> HHHHHHMAQDRKKVLVLGAGYAGLQTVTKLQKAISTEEAEITLINKNEYHYEATWLHEASAGTLNYEDVLYPVESVLKKDKVNFVQAEVTKIDRDAKKVETNQGIYDFDILVVALGFVSETFGIEGMKDHAFQIENVITARELSRHIEDKFANYAASKEKDDNDLSILVGGAGFTGVSFLGELTDRIPELCSKYGVDQ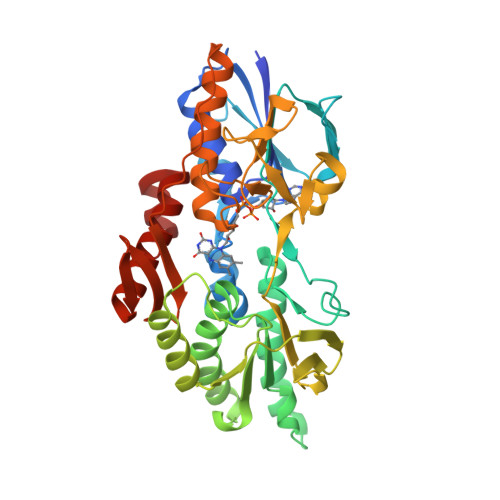NKVKITCVEAAPKMLPMFSEELVNHAVSYLEDRGVEFKIATPIVACNEKGFVVEVDGEKQQLNAGTSVWAAGVRGSKLMEESFEGVKRGRIVTKQDLTINGYDNIFVIGDCSAFIPAGEERPLPTTAQIAMQQGESVAKNIKRILNGESTEEFEYVDRGTVCSLGSHDGVGMVFGKPIAGKKAAFMKKVIDTRAVFKIGGIGLAFKKGKF>ATWTCINQQLNPKTNKWEDKRLLYSQAKAESNSHHAPLSDGKTGSSYPHWFTNGYDGNGKLIKGRTPIKFGKADCDRPPKHSQNGMGKDDHYLLEFPTFPDGHDYKFDSKKPKENPGPARVIYTYPNKVF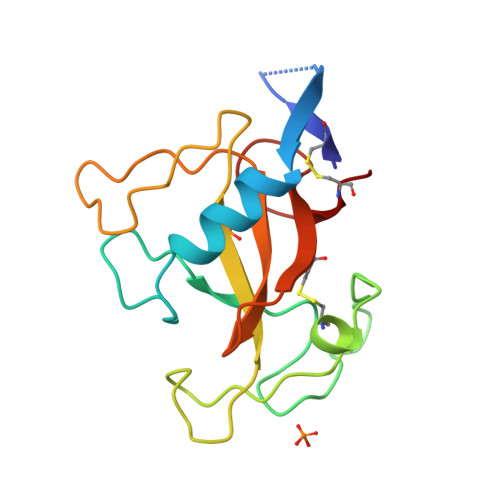CGIVAHQRGNQGDLRLCSH[2x]> GFFLYPHGFYGI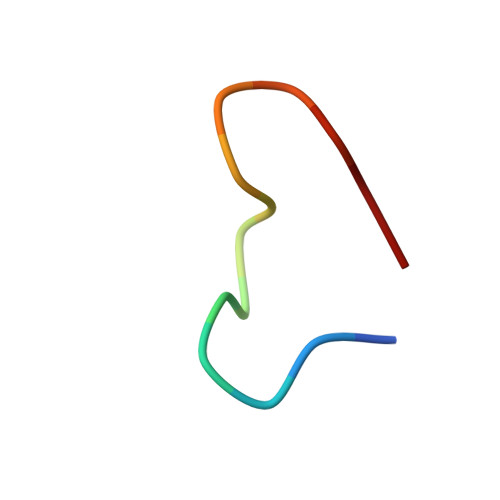VC> LPTSNPAQELEARQLGRTTRDDLINGNSASCADVIFIYARGSTETGNLGTLGPSIASNLESAFGKDGVWIQGVGGAYRATGGDNALPRGTSSAAIREMLGLFQQANTKCPDATLIAGGYSQGAALAAASIEDLDSAIRDKIAGTVLFGYTKNLQNRGRIPNYPADRTKVFCNTGDLVCTGSGIVA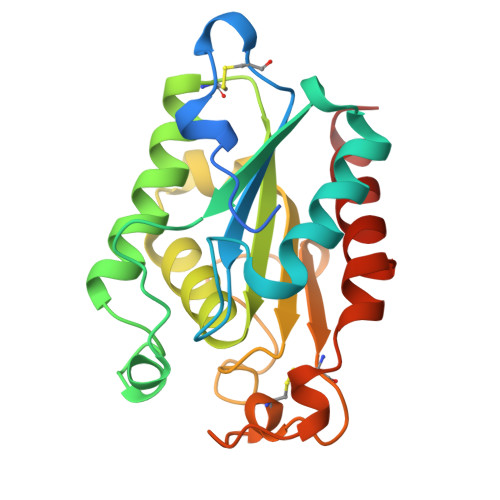APHLAYGPDARGPAPEFLIEKVRAVRGSA> ANVRLQHHHHHHHLEQGQNSVEIEAFGKRYFTDSVRNMKNADLYGGSIGYFLTDDVELALSYGEYHDVRGTYETGNKKVHGNLTSLDA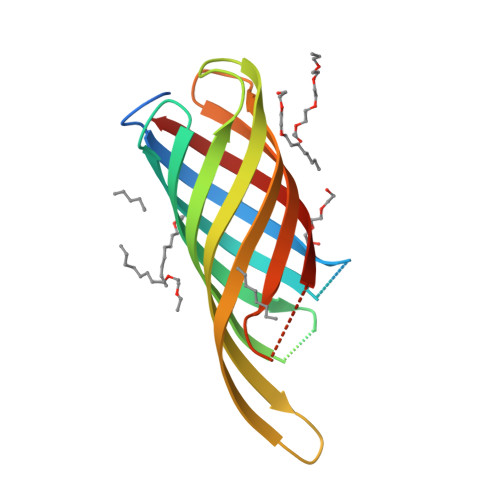IYHFGTPGVGLRPYVSAGLAHQNITNINSDSQGRQQMTMANIGAGLKYYFTENFFAKASLDGQYGLEKRDNGHQGEWMAGLGVGFNF> TVSTQTIGDESDPFLQNKRANDVIEQSLQLEKQRDKNEIKLLLLGADNSGKSTVLKQLKLLHGGSGGSGGTTGITETEFNIGSSKFKVLDAGGQRSERKKWIHCFEGITAVLFVLDMSDYNRMHESIMLFDTLLNSKWFKDTPFILFLNKIDLFEEKVKSMPIRKYFPDYQGR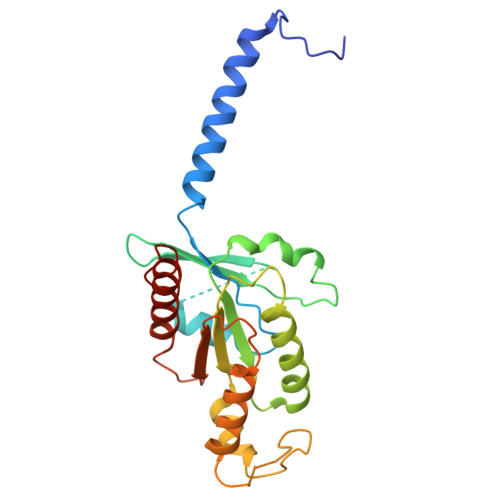VGDAEAGLKYFEKIFLSLNKTNKPIYVKRTCATDTQTAKFILSAVTDLIIQQNLKKIGII>GSGSGDVMRRRIATPEEVRLPLQHGWRREVRIKKGSHRWQGETWYYGPCGKRMKQFPEVIKYLSRNVVHS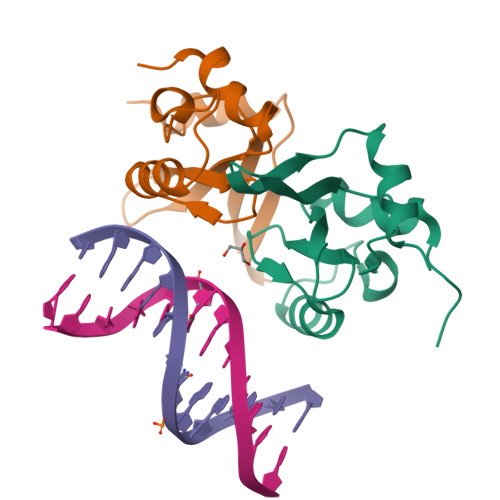VRREHFSFSPRMPVGDFFEERDTPEGLQWVQLSAEEIPSRIQAITGKRG[2x]> GGGGT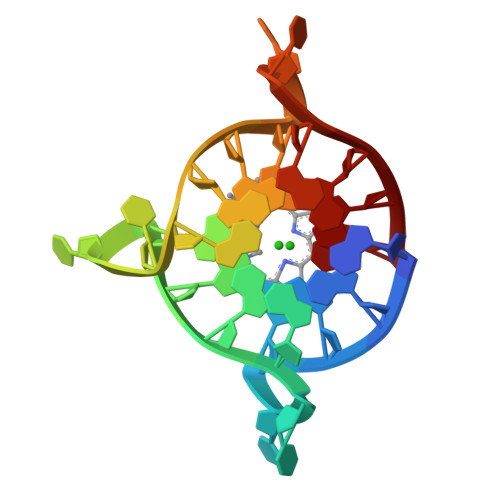TGGGGTTGGGGTTGGGG> MRLRISEAVVLFLLGAVAALIGDHSHVVTGTTVYHTDAVPFVWSSPFWFPILVGAATASLAELRLHLPAPRDGVTACQALGGVAAVVGTYVTTALVHAFPVVPVTALVAAAAAITWCVLGDGPGAAAGVVIAVIGPAVEIALVQLGVFAYHPDSDGLFGVAPFLAPLY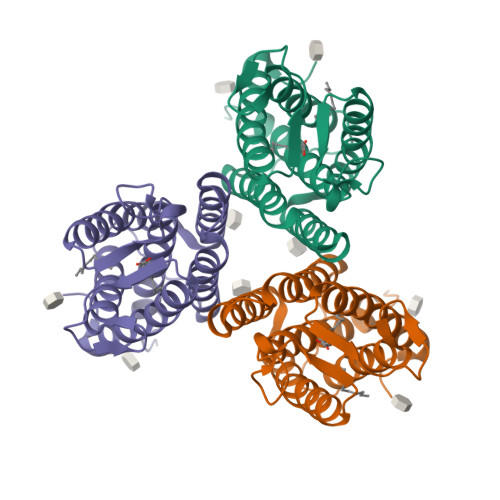FAFGVVAALLGELAVARRPQLGPPVADTVSRGPGAGHHHHHH>SMAGMSQRPPSMYWCVGPEESAVCPERAMETLNGAGDTGGKPSTRGGDPAARSRRTEGIRAAYRRGDRGGARDLLEEACDQCASQLEKGQLLSIPAAYGDLEMVRYLLSKRLVELPTEPTDDNPAVVAAYFGHTAVVQELLESLPGPCSPQRLLNWMLALACQRGHLGVVKLLVLTHGADPESYAVRKNEFPVIVRLPLYAAIKSGNEDIAIFLLRHGAYFCSYILLDSPDPSKHLLRKYFIEASPLPSSYPGKTALRVKWSHLRLPWVDLDWLIDISCQITELDLSANCLATLPSVIPWGLINLRKLNLSDNHLGELPGVQSSDEIICSRLLEIDISSNKLSHLPPGFLHLSKLQKLTASKNCLEKLFEEENATNWIGLRKLQELDISDNKLTELPALFLHSFKSLNSLNVSRNNLKVFPDPWACPLKCCKASRNALECLPDKMAVFWKNHLKDVDFSENALKEVPLGLFQLDALMFLRLQGNQLAALPPQEKWTCRQLKTLDLSRNQLGKNEDGLKTKRIAFFTTRGRQRSGTEAASVLEFPAFLSESLEVLCLNDNHLDTVPPSVCLLKSLSELYLGNNPGLRELPPELGQLGNLWQLDTEDLTISNVPAEIQKEGPKAMLSYLRAQLRKAEKCKLMKMIIVGPPRQGKSTLLEILQTGRAPQVVHGEATIRTTKWELQRPAGSRAKVESVEFNVWDIGGPASMATVNQCFFTDKALYVVVWNLALGEEAVANLQFWLLNIEAKAPNAVVLVVGTHLDLIEAKFRVERIATLRAYVLALCRSPSGSRATGFPDITFKHLHEISCKSLEGQEGLRQLIFHVTCSMKDVGSTIGCQRLAGRLIPRSYLSLQEAVLAEQQRRSRDDDVQYLTDRQLEQLVEQTPDNDIKDYEDLQSAISFLIETGTLLHFPDTSHGLRNLYFLDPIWLSECLQRIFNIKGSRSVAKNGVIRAEDLRMLLVGTGFTQQTEEQYFQFLAKFEIALPVANDSYLLPHLLPSKPGLDTHGMRHPTANTIQRVFKMSFVPVGFWQRFIARMLISLAEMDLQLFENKKNTKSRNRKVTIYSFTGNQRNRCSTFRVKRNQTIYWQEGLLVTFDGGYLSVESSDVNWKKKKSGGMKIVCQSEVRDFSAMAFITDHVNSLIDQWFPALTATESDGTPLMEQYVPCPVCETAWAQHTDPSEKSEDVQYFDMEDCVLTAIERDFISCPRHPDLPVPLQELVPELFMTDFPARLFLENSKLEHSEDEGSVLGQGGSGTVIYRARYQGQPVAVKRFHIKKFKNFANVPADTMLRHLRATDAMKNFSEFRQEASMLHALQHPCIVALIGISIHPLCFALELAPLSSLNTVLSENARDSSFIPLGHMLTQKIAYQIASGLAYLHKKNIIFCDLKSDNILVWSLDVKEHINIKLSDYGISRQSFHEGALGVEGTPGYQAPEIRPRIVYDEKVDMFSYGMVLYELLSGQRPALGHHQLQIAKKLSKGIRPVLGQPEEVQFRRLQALMMECWDTKPEKRPLALSVVSQMKDPTFATFMYELCCGKQTAFFSSQGQEYTVVFWDGKEESRNYTVVNTEKGLMEVQRMCCPGMKVSCQLQVQRSLWTATEDQKIYIYTLKGMCPLNTPQQALDTPAVVTCFLAVPVIKKNSYLVLAGLADGLVAVFPVVRGTPKDSCSYLCSHTANRSKFSIADEDARQNPYPVKAMEVVNSGSEVWYSNGPGLLVIDCASLEICRRLEPYMAPSMVTSVVCSSEGRGEEVVWCLDDKANSLVMYHSTTYQLCARYFCGVPSPLRDMFPVRPLDTEPPAASHTANPKVPEGDSIADVSIMYSEELGTQILIHQESLTDYCSMSSYSSSPPRQAARSPSSLPSSPASSSSVPFSTDCEDSDMLHTPGAASDRSEHDLTPMDGETFSQHLQAVKILAVRDLIWVPRRGGDVIVIGLEKDSGAQRGRVIAVLKARELTPHGVLVDAAVVAKDTVVCTFENENTEWCLAVWRGWGAREFDIFYQSYEELGRLEACTRKRR[2x]

Leucine Rich Repeat Kinase 1 and 2 (LRRK1 and LRRK2) are homologs in the ROCO family of proteins in humans. LRRK1 and LRRK2 have a similar domain organization: an N-terminal half containing Ankyrin (ANK) and Leucine Rich Repeats (LRR), and a catalytic C-terminal half containing the ROC–COR ROCO signature, followed by the kinase and a WD40 domain. Despite their shared domain architecture and involvement in intracellular trafficking, their disease associations are strikingly different: LRRK2 is involved in familial Parkinson’s disease while LRRK1 is linked to bone diseases. LRRK1 and LRRK2 use different mechanisms of autoinhibition, with LRRK1 having a second level of autoinhibition absent in LRRK2.

We imaged full-length LRRK1 in the presence of guanosine diphosphate (GDP). Surprisingly, this construct yielded almost exclusively dimers, of which we obtained a 4.6-Å structure. Each molecule in the dimer has the same conformation we observed in the monomer; however, the ANK domain is fully resolved in the dimer structure. Surprisingly, despite the similarities in their domain organization and the structures of the monomers, the LRRK1 dimer bears no resemblance to that of LRRK2. While LRRK2 forms a parallel dimer mediated by a single homotypic interaction involving its COR-B domain, LRRK1 forms an antiparallel dimer mediated by several homo- and heterotypic interactions. The ANK–LRR domains of each LRRK1 wrap around those of the other, making symmetrical contacts between the ANK:ANK and LRR:ANK domains. A major interaction interface is formed by the kinase C-lobe and LRR domains of one monomer and the opposite molecule’s ANK domain. In contrast to LRRK2, whose dimer is mediated entirely by the COR-B domain in its RCKW moiety, the LRRK1 dimer shows minimal direct interactions between RCKWs; the only contact seen in our structure is a homotypic interaction involving residues 1,263–1,265 in the kinase N-lobe. The main contact between the two LRRK1 monomers, and the most striking feature of the dimer, involves the ANK domains; each ANK domain contacts the opposite molecule’s kinase on both its N- and C-lobes, effectively blocking access to the kinase. Our structure suggests that the LRRK1 dimer uses the ANK domain to accomplish, in trans, the steric autoinhibition achieved by the LRR domain in the LRRK2 monomer.>[2x]SKEYHIDEEVGFALPNPQENLPDFYNDWMFIAKHLPDLIESGQLRERVEKLNMLSIDHLTDHKSQRLARLVLGCITMAYVWGKGHGDVRKVLPRNIAVPYCQLSKKLELPPILVYADCVLANWKKKDPNKPLTYENMDVLFSFRDGDCSKGFFLVSLLVEIAAASAIKVIPTVFKAMQMQERDTLLKALLEIASCLEKALQVFHQIHDHVNPKAFFSVLRIYLSG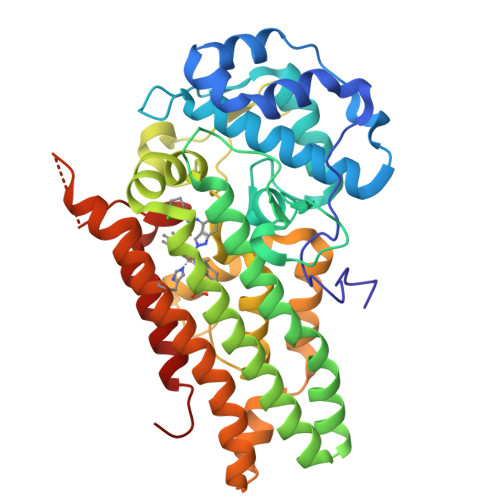WKGNPQLSDGLVYEGFWEDPKEFAGGSAGQSSVFQCFDVLLGIQQTAGGGHAAQFLQDMRRYMPPAHRNFLCSLESNPSVREFVLSKGDAGLREAYDACVKALVSLRSYHLQIVTKYILIPASQQPKENKTSEDPSKEEAKGTGGTDLMNFLKTVRSTTEKSLLKEG> GDYKEEEEIVEIDEEDAAMFEQYFKKSDDFNSLSGSYNLADKIMASIREKESQVEDMQDDEPLANEQNTSRGNISSGLKSGEGVALPEKVIKAYTTVGSILKTWTHGKLPKLFKVIPSLRNWQDVIYVTNPEEWSPHVVYEATKLFVSNLTAKESQKFINLILLERFRDNIETSEDHSLNYHIYRAVKKSLYKPSAFFKGFLFPLVETGCNVREATIAGSVLAKVSVPALHSSAALSYLLRLPFSPPTTVFIKILLDKKYALPYQTVDDCVYYFMRFRILDDGSNGE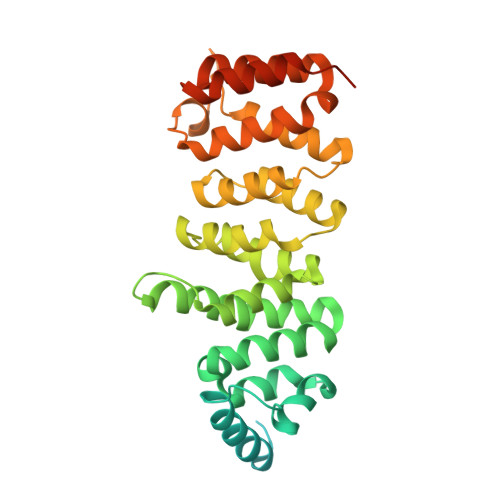DATRVLPVIWHKAFLTFAQRYKNDITQDQRDFLLETVRQRGHKDIGPEIRRELLAGASREFVDPQEANDDLMIDVN>[2x]GSMAAAGRRILADWVTGKVTKVQNWTDALFSLTVHAPVLPFTAGQFTKLGLEIDGERVQRAYSYVNSPDNPDLEFYLVTVVYTNDAGEVVKGKLSPRLAALKPGDEVQVVSEAAGFFVLDEVPHCETLWMLATGTAIGPYLSILRLGKDLDRFKNLVLVHAARYAADLSYLPLMQELEKRYEGKLRIQTVVSRETAAGSLTGRIPALIESGELESTIGLPMNKETSHVMLCGNPQMVRDTQQLLKET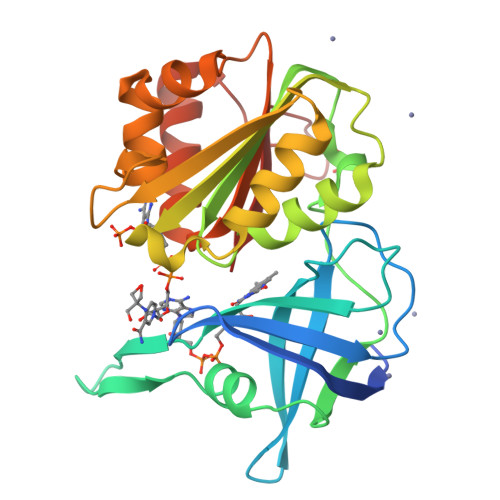RQMTKHLRRRPGHMTAEHY>GVPAEGAFTEDFQGLRAEVETISKELELLDRELCQLLLEGLEGVLRDQLALRALEEALEQGQSLGPVEPLDGPAGAVLECLVLSSGMLVPELAIPVV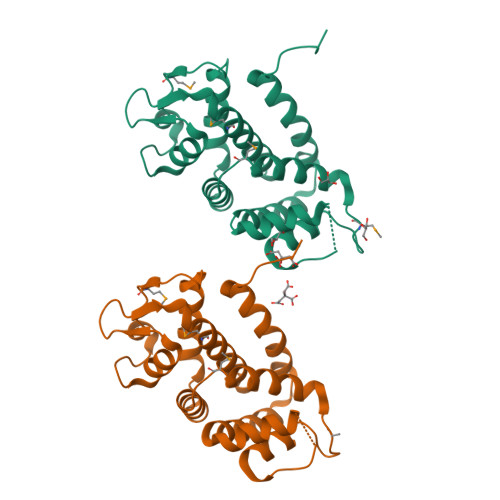YLLGALTMLSETQHKLLAEALESQTLLGPLELVGSLLEQSAPWQERSTMSLPPGLLGNSWGEGAPAWVLLDECGLELGEDTPHVCWEPQAQGRMCALYASLALLSGLSQEPH[2x]> PT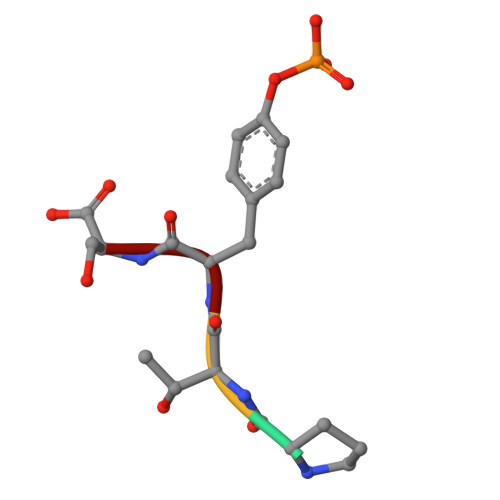YS>GAMGSSRKSKAELQSEERKRIDELIESGKEEGMKIDLIDGKGRGVIATKQFSRGDFVVEYHGDLIEITDAKKREALYAQDPSTGCYMYYFQYLSKTYCVDATRETNRLGRLINHSKCGNCQTKLHDIDGVPHLILIASR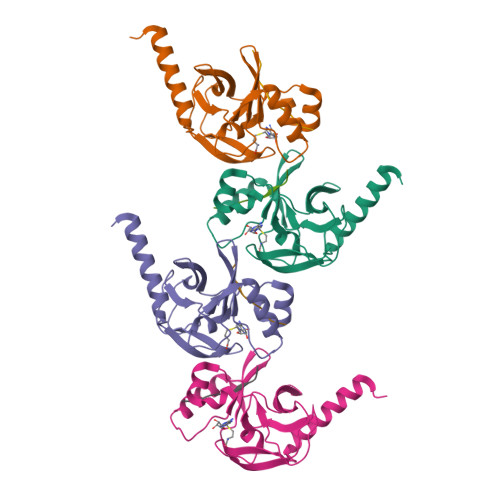DIAAGEELLYDYGDRSKASIEAHPWLKH[4x];>AKRHRKVLRD[4x]> TTPLVHVASVEKGRSYEDFQKVYNAIALKLREDDEYDNYIGYGPVLVRLAWHTSGTWDKHDNTGGSYGGTYRFKKEFNDPSNAGLQNGFKFLEPIHKEFPWISSGDLFSLGGVTAVQEMQGPKIPWRCGRVDTPEDTTPDNGRLPDADKDADYVRTFFQRLNMNDREVVALMGAHALGKTHLKNSGYEGPWGAANNVFTNEFYLNLLNEDWKLEKNDANNEQWDSKSGYMMLPTDYSLIQDPKYLSIVKEYANDQDKFFKDFSKAFEKLLENGITFPKD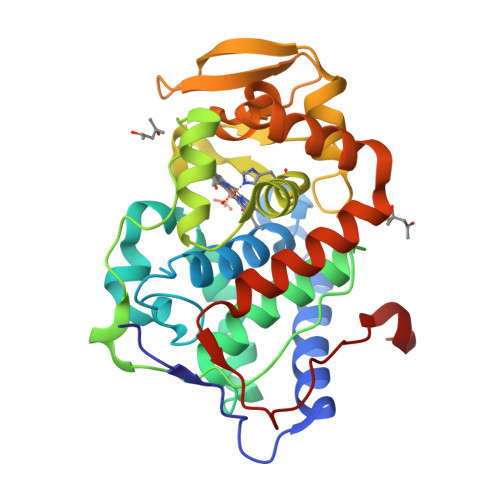APSPFIFKTLEEQGL> MKFPAFSYRAPASLQEVIQVLA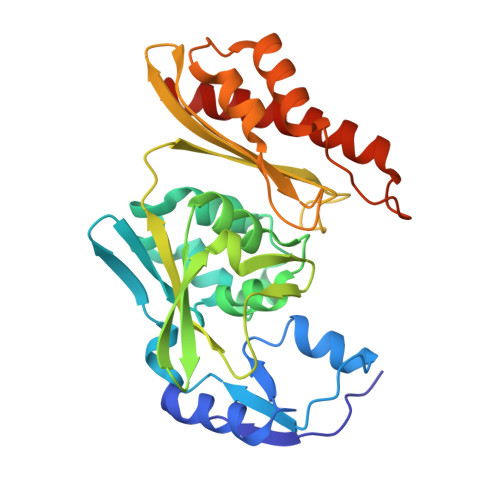DDPDARIIAGGQSLLPLLAFRLVYPSCLVDLRNVSELFEISQSAGILSVGAMVTHFRNKTDPTVAKCVPILPKVLAHVAHQAVRNRGTLGGSLAHADAGAEMPFLMATLGATMYIASSAGVRSVSATDFMKGHYFTDLEAGEVLVRVEIPIPALHWEFDEYARRKGDYALVMAAAGLSMQGGRCVAARIALGAVEERAHQAIRANDFLVGKVIDESTAATAAELATEGLEPRSDIHGSRDLRLSLAKAITQRVILKAAQGAMYAGA N-[(5S,7R,8S,9S,10R)-8,9,10-trihydroxy-7-(hydroxymethyl)-2,4-dioxo-6-oxa-1,3-diazaspiro[4.5]dec-3-yl]acetamide 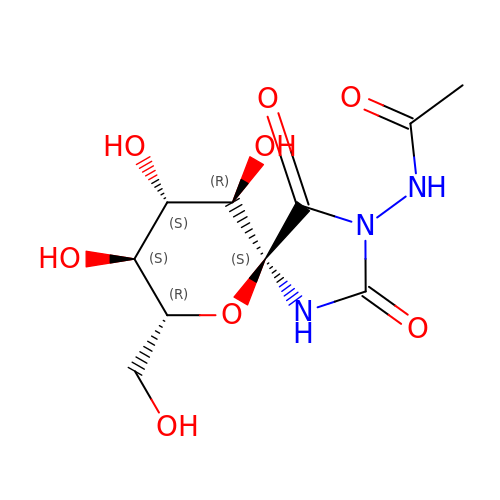| C10 H15 N3 O8 | MAHIOGAAEAWGLR-UTAYWCBXSA-N> MIDTWLAQWGLRLPSSNDATLRLQPAEGPELVMERLEGGWLFVVELGLVPSGLPLGVILQLLQVNSPFSSLAPVKLAADDAGRLVLWAEARDGVDDVDALNRLHDRLREGHSRLVPLLEPTGELVPA;> GSSLRQEPSGQGLGVALKSTPGILSGKLPESVSDVRFSSPQGQGESRTLTDSAGPRQITLRQFENGVTELQLSRPPLTSLVLSGGGAKGAAYPGAMLALEEKGMLDGIRSMSGSSAGGITAALLASGMSPAAFKTLSDKMDLISLLDSSNKKLKLFQHISSEIGASLKKGLGNKIGGFSELLLNVLPRIDSRAEPLERLLRDETRKAVLGQIATHPEVARQPTVAAIASRLQSGSGVTFGDLDRLSAYIPQIKTLNITGTAMFEGRPQLVVFNASHTPDLEVAQAAHISGSFPGVFQKVSLSDQPYQAGVEWTEFQDGGVMINVPVPEMIDKNFDSGPLRRNDNLILEFEGEAGEVAPDRGTRGGALKGWVVGVPALQAREMLQLEGLEELREQTVVVPLKSERGDFSGMLGGTLNFTMPDEIKAHLQERLQERVGEHLEKRLQASERHTFASLDEALLALDDSMLTSVAQQNPEITDGAVAFRQKARDAFTELTVAIVSANGLAGRLKLDEAMRSALQRLDALADTPERLAWLAAELNHADNVDHQQLLDAMRGQTVQSPVLAAALAEAQRRKVAVIAENIRKEVIFPSLYRPGQPDSNVALLRRAEEQLRHATSPAEINQALNDIVD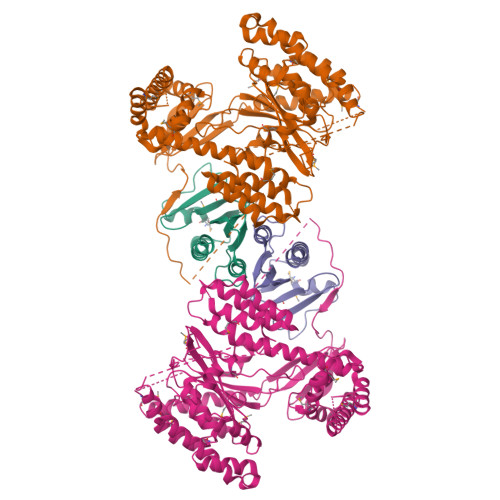NYSARGFLRFGKPLSSTTVEMAKAWRNKEFT>[2x]GMNHNYVEVKYPAIFRDEGTYWDVRFPDVPAAQTFGA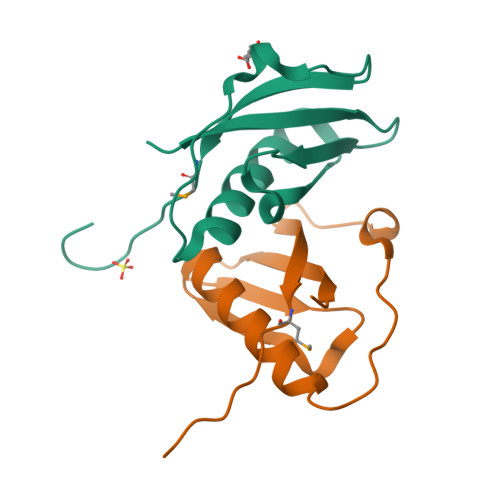SVQVAADNAANALAIALFEQSLPPASDPQYWRLASTEFVVWITMADVQFGPGADTPEPMN> GCPQEDSDIAFLIDGSGSIIPHDFRRMKEFVSTVMEQLKKSKTLFSLMQYSEEFRIHFTFKEFQNNPNPRSLVKPITQLLGRTHTATGIRKVVRELFNITNGARKNAFKILVVITDGEKFGDPLGYED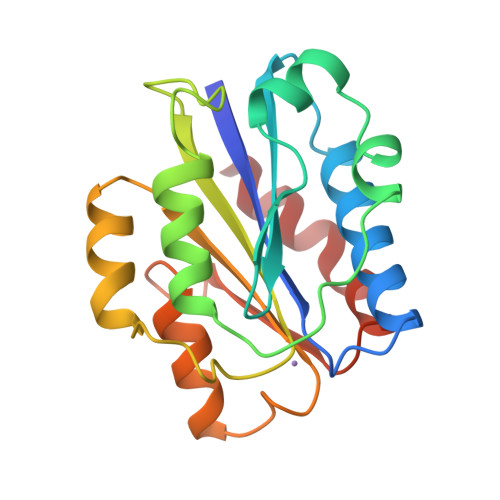VIPEADREGVIRYVIGVGDAFRSEKSRQELNTIASKPPRDHVFQVNNFEALKTIQNQLREKIFA>[2x]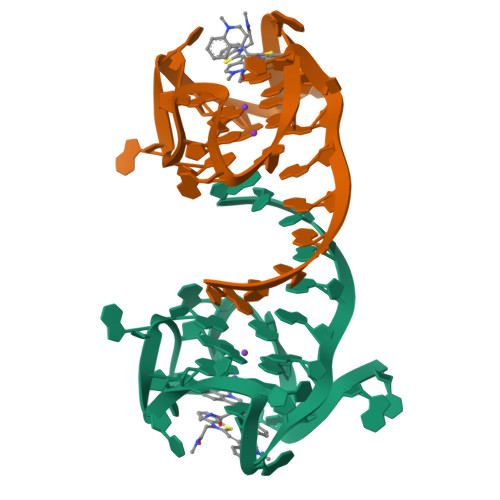AUCGAGGGAGUGGUGAGGAUGAGGCGAU> GPHMEDENILRNAVNLQVLKFHYPEIESIIDIASHVAVYQFDVGS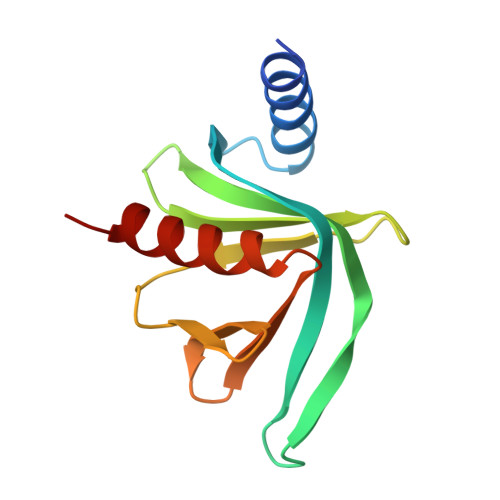QKWLKTSIEGTFFLVKDQRARVGYVILNRNSPENLYLFINHPSNVHLVDRYLIHRTENQHVVGLWMFDPNDMSRIFNIVKESLLR>MGSSHHHHHHSSGLVPRGSHMPSYTVTVATGSQEHAGTDDYIYLSLVGSAGCSEKHLLDKGSFERGAVDSYDVTVDEELGEIQLVRIEKRKYGSNDDWYLKYITLKTPHGDYIEFPCYRWITGDVEVVLRDGRAKLARDDQIHILKQHRRKELETRQKQYRWMEWNPGFPLSIDAKCHKDLPRDIQFDSEKGVDFVLNYSKAMENLFINRFMHMFQSSWNDFADFEKIFVKISNTISERVMNHWQEDLMFGYQFLNGANPVLIRRCTELPEKLPVTTEMVECSLERQLSLEQEVQQGNIFIVDFELLDGIDANKTDPCTLQFLAAPICLLYKNLANKIVPIAIQLNQIPGDENPIFLPSDAKYDWLLAKIWVRSSDFHVHQTITHLLRTHLVSEVFGIAMYRQLPAVHPIFKLLVAHVRFTIAINTKAREQLICECGLFDKANATGGGGHVQMVQRAMKDLTYASLCFPEAIKARGMESKEDIPYYFYRDDGLLVWEAIRTFTAEVVDIYYEGDQVVEEDPELQDFVNDVYVYGMRGRKSSGFPKSVKSREQLSEYLTVVIFTASAQHAAVNFGQYDWASWIPNA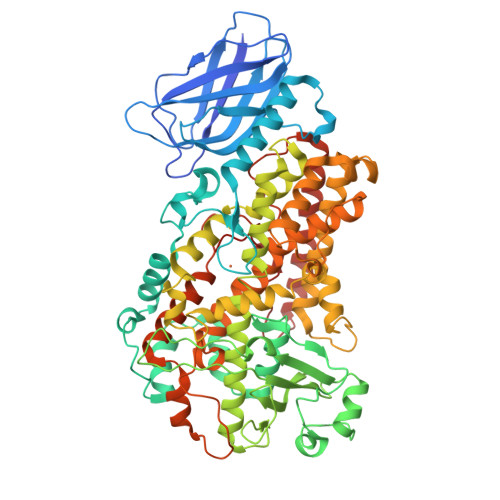PPTMRAPPPTAKGVVTIEQIVDTLPDRGRSCWHLGAVWALSQFQENELFLGMYPEEHFIEKPVKEAMARFRKNLEAIVSVIAERNENLQLPYYYLDPDRIPNSVAI[2x]> DNPPDPTPAKFFVPIPSHSWAHGTNTSEPTNTLRLDGGVVGVGRSDDIGTSDTAISGIIGVYGLLKPF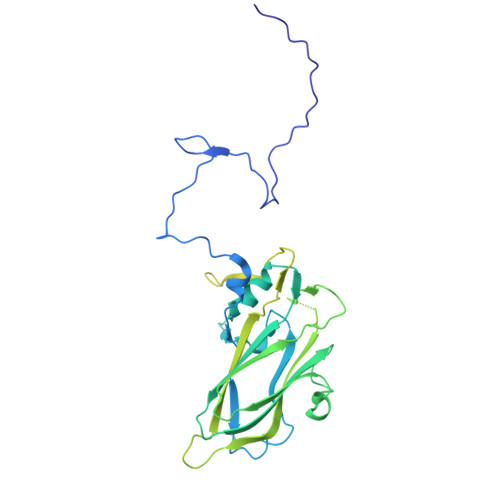DWNANDTGRNVGGHLLWSMPVHPQVDKDQVIQVMTQSKLTQYYLPPISVVSSLYAYTRGSIKYKFLFGNNPRHNARLLVAYIPGISSDNRLTLERARNSAHVVFSLNEVSEFVFTVPYITDTMWWPRKYGGPQAAGEFVAPSYICMFILNPLVAMESVPSIVTIVPMIAAGDDFEVAVPAQPAVGLSRNIDVIYPKDSIISFKSGYFPVYVGSWHSFFDSTKAILRYGAVSDHIAQLGNIPANVNRKAFWIVVGDTIKFKTKLDKINGTEWFIPEGEYTLGYGVVWRDGAYAYMVPYPLTPLGEKIAQYTASLLASNTAISQIRPYIPDYIVDSAASKDNILWSPIEDRLRAQTEWVMAEPE> MEEIQGYDVEFDPPLESKYECPICLMALREAVQTPCGHRFCKACIIKSIRDAGHKC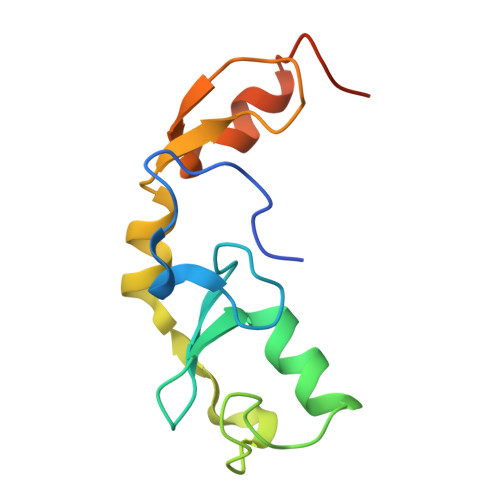PVDNEILLENQLFPDNFAKREILSLMVKCPNEGCLHKMELRHLEDHQAHCEFALLEHHHHHH> GAGCAGACGTGACGAGACTCA;> TCGTCA;> TCTGAGTC;> CGTCTGC

In this work, we exhaustively probe the ability of all 36 immobile HJ sequences to form DNA crystals in two different designed systems. Three separate self-assembling DNA crystal systems are described in this report: the “4 × 5” and “4 × 6” designs (collectively referred to as the 4 × N systems), and a third construct with a “scrambled” sequence variant of the 4 × 6 lattices. Self-assembly was mediated by three constituent oligonucleotides: (S1) containing four sequence repeats of either 5 or 6 bases; (S2) composed of 21 bases containing complementary regions to both (S1); and (S3) which forms the second junction crossover. The HJ serves as the fundamental component at the core of each unit, and the ultimate assembly of the full lattice is facilitated by the complementary 2-base sticky ends that tail each duplex.

Each asymmetric unit could be defined as either a HJ containing 10 and 11 bp on each arm, or as a 21-bp linear duplex. In parallel, we employed the previously reported J1 4 × 6 system (3.05 Å), with P32 symmetry. Seventeen of the 36 junctions successfully crystallized, a 47% success rate. Unlike the 4 × 5 motif, nearly all of the 4 × 6 junction sequences had a strong preference for crystallization in buffers containing ≥2.0 M salts (e.g., LiCl, Li2SO4, KCl, and NaCl), with the majority preferring slightly basic pH conditions in cacodylic acid. The average cell constants for the P32 crystals were a = b = 68.29 Å c = 55.68 Å. The c-axis, in particular, was ~5 Å shorter, and had a much larger degree of variability (σ = 1.97), than those that crystallized using the 4 × 5 motif. The broad range of the short axis spanned from 52.77 to 60.36 Å, and we posit that the flexible axis lengths could be responsible for rendering a larger number of junctions fatal than the 4 × 5 system. However, in the majority of the crystal structures reported here, the cacodylate anion indeed fits best into the electron density map of our X-ray structures, due to the presence of sodium cacodylate in the crystallization solution.>[2x]DHNFMRREIKIEGDLVLGGLFPINEKGTGTEECGRINEDRGIQRLEAMLFAIDEINKDNYLLPGVKLGVHILDTCSRDTYALEQSLEFVRASLTKVDEAEYMCPDGSYAIQENIPLLIAGVIGGSYSSVSIQVANLLRLFQIPQISYASTSAKLSDKSRYDYFARTVPPDFYQAKAM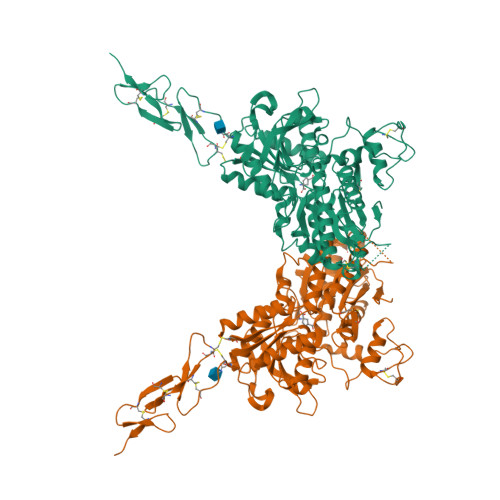AEILRFFNWTYVSTVASEGDYGETGIEAFEQEARLRNICIATAEKVGRSNIRKSYDSVIRELLQKPNARVVVLFMRSDDSRELIAAANRVNASFTWVASDGWGAQESIVKGSEHVAYGAITLELASHPVRQFDRYFQSLNPYNNHRNPWFRDFWEQKFQCSLQNKRNHRQVCDKHLAIDSSNYEQESKIMFVVNAVYAMAHALHKMQRTLCPQTTKLCDAMKILDGKKLYKEYLLKIQFTAPFNPNKGADSIVKFDTFGDGMGRYNVFNLQQTGGKYSYLKVGHWAETLSLDVDSIHWSRNSVPTSQCSDPCAPNEMKNMQPGDVCCWICIPCEPYEYLVDEFTCMDCGPGQWPTADLSGCYNLPEDYIKWEDALVPR>[4x]GGSGSSPSLEQDDGDEETSVVIV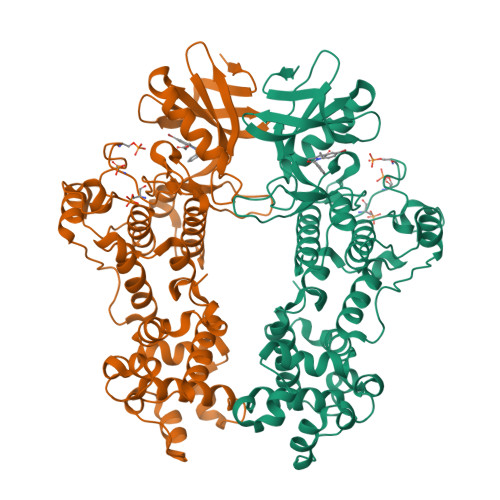GKISFCPKDVLGHGAEGTIVYRGMFDNRDVAVKRILPECFSFADREVQLLRESDEHPNVIRYFCTEKDRQFQYIAIELCAATLQEYVEQKDFAHLGLEPITLLQQTTSGLAHLHSLNIVHRDLKPHNILISMPNAHGKIKAMISDFGLCKKLAVGRHSFSRRSGVPGTEGWIAPEMLSEDCKENPTYTVDIFSAGCVFYYVISEGSHPFGKSLQRQANILLGACSLDCLHPEKHEDVIARELIEKMIAMDPQKRPSAKHVLKHPFFWSLEKQLQFFQDVSDRIEKESLDGPIVKQLERGGRAVVKMDWRENITVPLQTDLRKFRTYKGGSVRDLLRAMRNKKHHYRELPAEVRETLGSLPDDFVCYFTSRFPHLLAHTYRAMELCSHERLFQPYYFHEPPEPQPPVTPDAL> AQSVPYGVSQIKAPALHSQ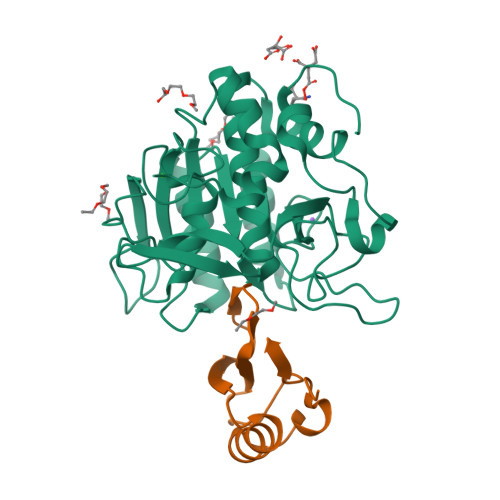GYTGSNVKVAVIDSGIDSSHPDLKVAGGASMVPSETNPFQDNNSHGTHVAGTVAALNNSIGVLGVAPSASLYAVKVLGADGSGQYSWIINGIEWAIANNMDVINMSLGGPSGSAALKAAVDKAVASGVVVVAAAGNEGTSGSSSTVGYPGKYPSVIAVGAVDSSNQRASFSSVGPELDVMAPGVSIQSTLPGNKYGAYNGTSMASPHVAGAAALILSKHPNWTNTQVRSSLENTTTKLGDSFYYGKGLINVQAAAQHHHHHH;> MKTEWPELVGKSVEEAKKVILQDKPAAQIIVLPVGTIVTMEARIDRVRLFVDRLDNIAQVPRVG>MSQLDLLNIVHRPRRLRRTAAL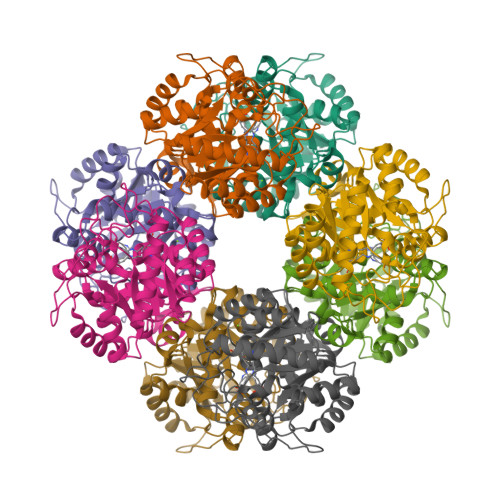RNLVQENTLTVNDLVFPLFVMPGTNAVEEVSSMPGSFRFTIDRAVEECKELYDLGIQGIDLFGIPEQKTEDGSEAYNDNGILQQAIRAIKKAVPELCIMTDVALDPFTPFGHDGLVKDGIILNDETVEVLQKMAVSHAEAGADFVSPSDMMDGRIGAIREALDETDHSDVGILSYAAKYASSFYGPFRDALHSAPQFGDKSTYQMNPANTEEAMKEVELDIVEGADIVMVKPGLAYLDIVWRTKERFDVPVAIYHVSGEYAMVKAAAAKGWIDEDRVMMESLLCMKRAGADIIFTYYAKEAAKKLR[2x]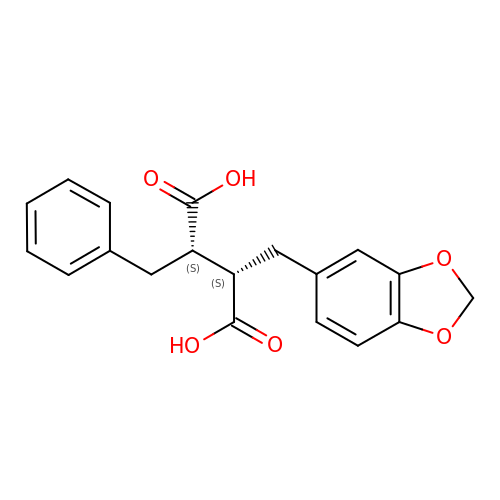2-BENZO[1,3]DIOXOL-5-YLMETHYL-3-BENZYL-SUCCINIC ACID | C19 H18 O6 | ASEJDWRSZYAIOT-GJZGRUSLSA-N>GSTGSVEQDQPAPIPENSEMDQAKEKAKIAVSKYMSKVLDGVHQHLQKKNHSKIVDLFKELEAIKQQTI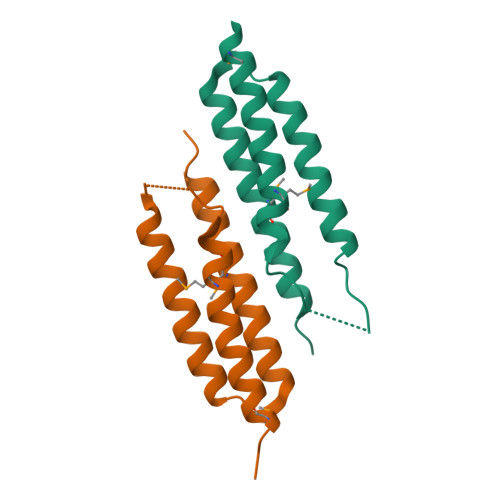FDIDNAKTEVEIDNLVHDAFSKMNATVAKFQKGLETNT[2x]> NLYFQSNAMKHCPITYEKISDQENYSQRGLHLLSPQLKNLSPLDLSADEQRQEAIARVGKMSVQGVQKKLSAKL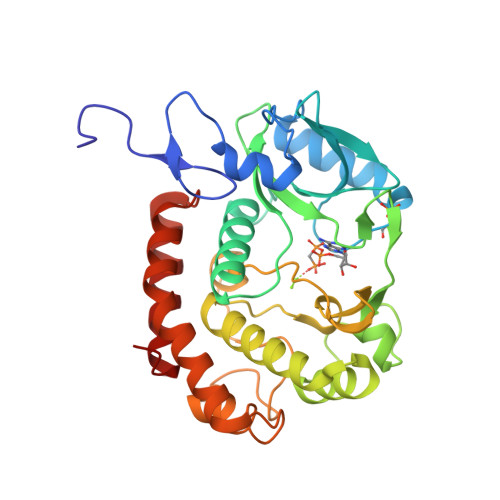KIKEGCFEIVDQYGQYILKPQSDIYPELPENEAITMTLAKTIGLEVPVHGLVYSKDNSLTYFIKRFDRIGHNKKLALEDFAQLSGEDRHTKYKSSMEKVIAVIEQFCTFPKIEFVKLFKLTLFNFLVGNEEMHLKNFSLITKDRKISISPAYDLLNSTIAQKNTKEELALPLKGKKNNLTKSDFLKYFAIEKLGLNQNVIDGIVQEFHQVIPKWQELIGFSFLSQEMQEKYLELLEQRCKRLNFFD>GPGSSHWTSKVHESVIGRNPEGQLGFELKGGAEN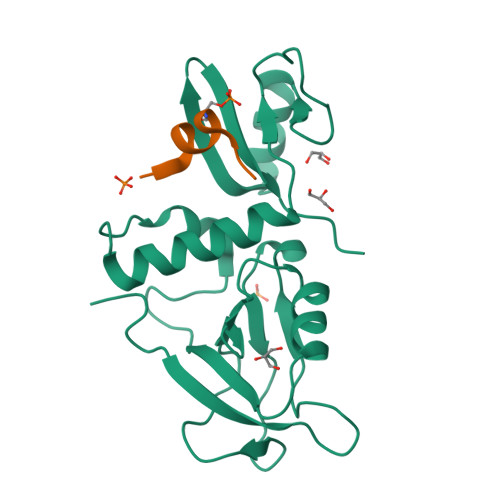GQFPYLGEVKPGKVAYESGSKLVSEELLLEVNETPVAGLTIRDVLAVIKHCKDPLRLKCVKQGGIVDKDLRHYLNLRFQKGSVDHELQQIIRDNLYLRTVPCTTRPHKEGEVPGVDYIFITVEEFMELEKSGALLESGTYEDNYYGTPKPPAEPAPLLNVTDQILPGATPSAEGKRKRNKSVTNMEKASIEPPEEEEEER[2x];>IRSHSYLRAVSEVS[2x]> GSQTKPLPALKLALEYIVPCMNKHGICVVDDFLGKETGQQIGDEVRALHDTGKFTDGQLVSQKSDSSKDIRGDKITWIEGKEPGCETIGLLMSSMDDLIRHCNGKLGSYKINGRTKAMVACYPGNGTGYV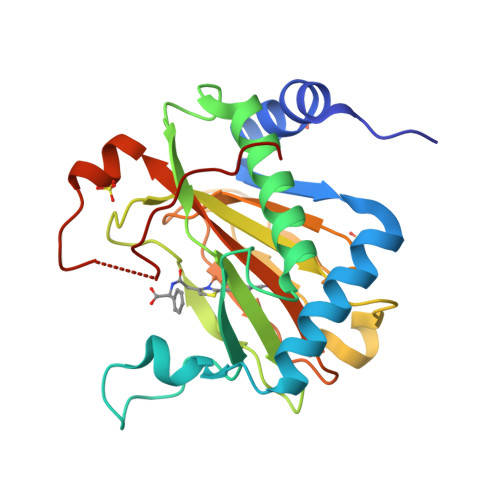RHVDNPNGDGRCVTCIYYLNKDWDAKVSGGILRIFPEGKAQFADIEPKFDRLLFFWSDRRNPHEVQPAYATRYAITVWYFDADERARAKVKYLTGEKGLRVELNKPSD>CGCTATAATGCG[2x];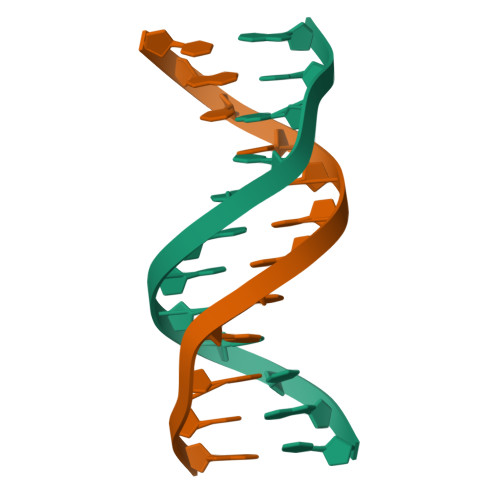>[2x]CGCATTATAGCG>GLIVDTRDVEERVHVMRKTKLAPTVAHGVFNPEFGPAALSNKDPRLNEGVVLDEVIFSKHKGDTKMSAEDKALFRRCAADYASRLHSVLGTANAPLSIYEAIKGVDGLDAMEPDTAPGLPWALQGKRRGALIDFENGTVGPEVEAALKLMEKREYKFACQTFLKDEIRPMEKVRAGKTRIVDVLPVEHILYTRMMIGRFCAQMHSNNGPQIGSAVGCNPDVDWQRFGTHFAQYRNVWDVDYSAFDANHCSDAMNIMFEEVFRTEFGFHPNAEWILKTLVNTEHAYENKRITVEGGMPSGCSATSIINTILNNIYVLYALRRHYE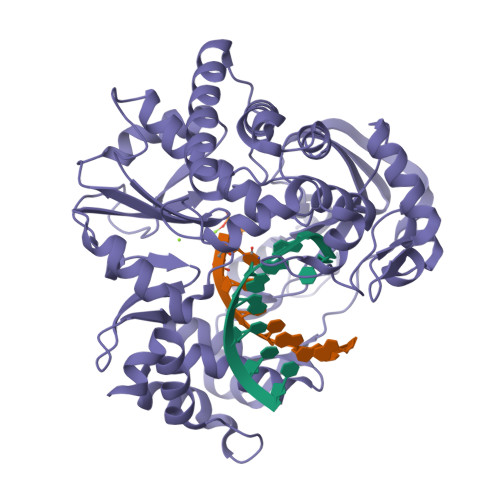GVELDTYTMISYGDDIVVASDYDLDFEALKPHFKSLGQTITPADKSDKGFVLGHSITDVTFLKRHFHMDYGTGFYKPVMASKTLEAILSFARRGTIQEKLISVAGLAVHSGPDEYRRLFEPFQGLFEIPSYRSLYLRWVNAVCGDAAALEHH[2x]>[2x]NEDICFIAGIGDTNGYGWGIAKELSKRNVKIIFGIWPPVYNIFMKNYKNGKFDNDMIIDKDKKMNILDMLPFDASFDTANDIDEETKNNKRYNMLQNYTIEDVANLIHQKYGKINMLVHSLANAKEVQKDLLNTSRKGYLDALSKSSYSLISL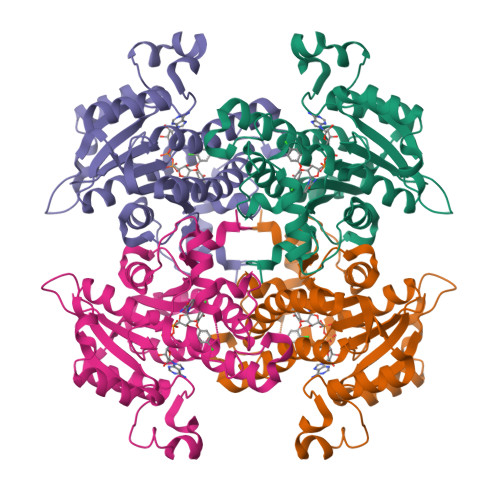CKYFVNIMKPQSSIISLTYHASQKVVPGYGGGMSSAKAALESDTRVLAYHLGRNYNIRINTISAGPLKSRAATAINKLNNTYENNTNQNKNRNRHDVHNIMNNSGEKEEKKISASQNYTFIDYMIEYSEKYAPLRQKLLSTDIGSVASFLLSRESRAITGQTIYVDNGLNIMFLPD> GHMQIGWRREGIKYRRNELFLDVLESVNLLMSPQGQVLSAHVSGRVVMKSYLSGMPECKFGMNDKIVIEKQGKGTADETSKSGKQSIAIDDCTFHQCVRLSKFDSERSISFIPPDGEFELMRYRTTKDIILPFRVIPLVREVGRTKLEVKVVI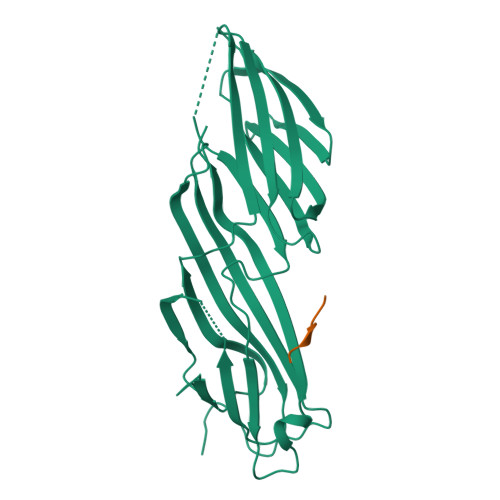KSNFKPSLLAQKIEVRIPTPLNTSGVQVICMKGKAKYKASENAIVWKIKRMAGMKESQISAEIELLPTNDKKKWARPPISMNFEVPFAPSGLKVRYLKVFEPKLNYSDHDVIKWVRYIGRSGIYETRC;> LYCYEQLNDEE> MGTRDDEYDYLFKVVLIGDSGVGKSNLLSRFTRNEFNLESKSTIGVEFATRSIQVDGKTIKAQIWDTAGQERYRAITSAYYRGAVGALLVYDIAKHLTYENVERWLKELRDHADSNIVIMLVGNKSDLRHLRAVPTDEARAFAEKNGLSFIETSALDSTNVEAAFQTILTEIY;> GAMAAKFRASNIMPSSSFHMSPTSNEDLRKIPDSNPFDATAGYRSLTYEEVLQELVKHKELLRRKDTHIRELEDYIDNLLVRVMEETPS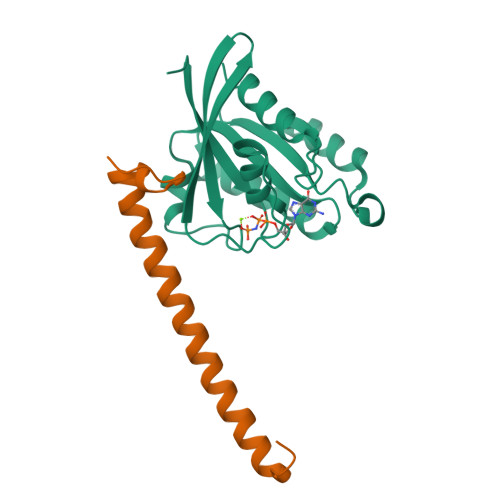ILRVPYEPSRKAGKFSNS> MNIKALLLITSAIFIS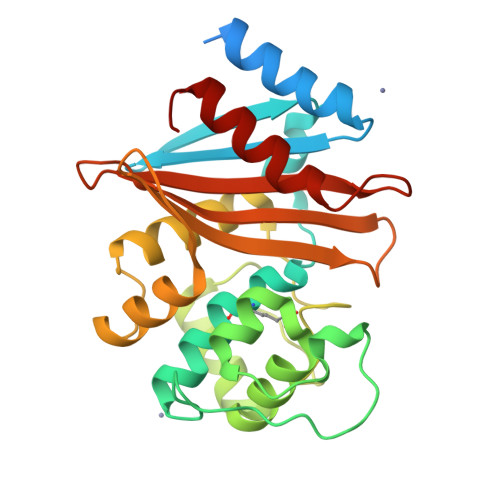ACSPYIVTANPNHSASKSDVKAEKIKNLFNEAHTTGVLVIQQGQTQQSYGNDLARASTEYVPASTFKMLNALIGLEHHKATTTEVFKWDGKKRLFPEWEKDMTLGDAMKASAIPVYQDLARRIGLELMSKEVKRVGYGNADIGTQVDNFWLVGPLKITPQQEAQFAYKLANKTLPFSQKVQDEVQSMLFIEEKNGNKIYAKSGWGWDVNPQVGWLTGWVVQPQGNIVAFSLNLEMKKGIPSSVRKEITYKSLEQLGIL>GSSQAKPPTRLFRGLNLSEEFTKGLIDQANAMIANTTERLFTDHSPEAFKQIKLNDLSKMSGRTNASTTTEIKLVKETWDSNVIFEMLDPDGLLHSKQVGRHGEGTASAFSVYLPEDVALVPVKVTLDGKTQKGENRYVFTFVAVKSPDFTP[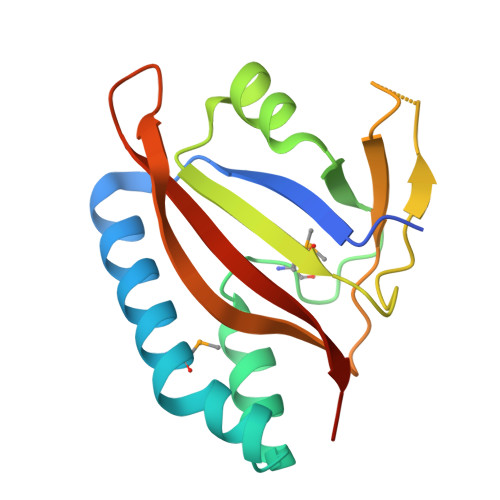4x]> AAAAAAA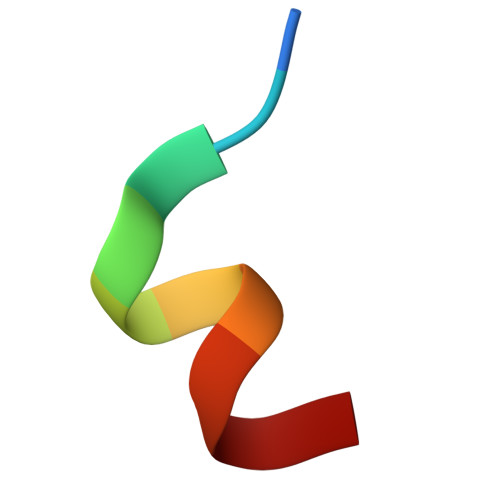AAA Growth-factor receptor-bound protein 2 (Grb2) is an adaptor protein that has an SH3-SH2-SH3 domain architecture. The Grb2 SH2 domain mediates activation of the Ras pathway through binding to phosphotyrosyl motifs on either growth factor receptors such as epidermal growth factor receptor or other adaptor proteins such as Shc. Grb2 SH2 specifically binds to the pY-X-N-X consensus sequence where X is any amino acid; however, it binds to pY-(L/V)-N-(V/P) with higher affinity. A number of signaling molecules such as Grb2 and phosphatidylinositol 3-kinase (PI3K) bind to the cytoplasmic region of CD28 and activate CD28-mediated costimulatory signaling.

In this study, we report the crystal structure of Grb2 SH2 in complex with a CD28-derived peptide consisting of 8 amino acids, including the pY-M-N-M sequence, at a resolution of 1.35 Å. In general, the folds of the Grb2 SH2 domain were essentially the same as those previously reported; consisting of a central, antiparallel β-sheet flanked by 2 α-helices. The phosphorylated CD28 peptide binds to the Grb2 SH2 recognition site across the exposed edge of the central β-sheet. The phosphate moiety of the phosphotyrosine (pTyr191pep, the amino acid residues of the CD28-derived peptide are denoted with a “pep” suffix hereafter) directly interacts with the side chains of Arg67, Arg86, Ser88, Ser90, and Ser96. The side-chain of Asn193pep at the pY+2 position forms a pair of hydrogen bonds with the main-chain amide and carbonyl groups of Lys109. The 2 methionine residues, which are unique to the CD28-derived peptide, appear to contribute to the binding mainly through hydrophobic interactions. The peptide adopts a bent conformation similar to the type-I β-turn, which is the canonical conformation of peptides bound to Grb2 SH2. However, the hallmark hydrogen bond between the main-chain oxygen of pY and the main-chain nitrogen of the pY+3 residue (Met194pep in our structure) is not formed. Consequently, the CD28-derived peptide is slightly lifted away from Grb2 SH2, making it a more “twisted” conformation than a canonical type-I β-turn. A very strong electron density, which was interpreted as a cadmium ion, was observed between 2 molecules in the crystal lattice.

> GSPEFWFFGKIPRAKAEEMLSKQRHDGAFLIRESESAPGDFSLSVKFGNDVQHFKVLRDGAGKYFLWVVKFNSLNELVDYHRSTSVSRNQQIFLRDIE;> SDYMNMTP>[16x]SEEVVENPTIQKDVLECNVKTTEVVGDIILKPANNSLKITEEVGHTDLMAAYV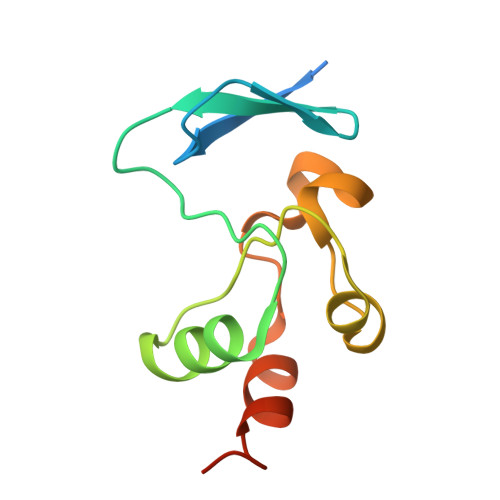DNSSLTIKKPNELSRVLGLKTLATHGLAAVNSVPWDTIANYAKPFLNKVVST>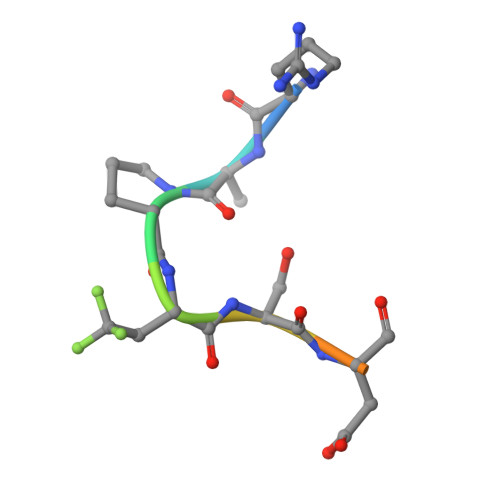 RAPXSDITN Earlier work in 2005 revealed that GRETCHEN HAGEN 3 (GH3) proteins, known for their role in forming IAA-amides with amino acids (IAA-AAs), also exhibit in vitro sensitivity to PAA. To investigate the spectrum activity of GH3 enzymes to form PAA amino acid conjugates, recombinant AtGH3.6 and AtGH3.17 enzymes were tested with PAA using a bacterial assay. Nonetheless, AtGH3.6 predominantly conjugated PAA with Asp and AtGH3.17 with Glu. To understand the basis for amino acid specificity in GH3s, we solved the crystal structure of AtGH3.6 in the presence of AMP only or AMP together with aspartate, up to 1.74 Å resolution.

Superposition of both structures did not reveal rearrangement in the presence of amino acid (aspartate) ligand in the active site. Binding affinities for AtGH3.6 were analysed by MST. Affinities for IAA and PAA were similar and at around 60 µM concentration. The superposition of AtGH3.6 with AtGH3.5 shows the conservation of the amino acid binding site and, thus, similar specificity. Our attempts to obtain structures with bound products IAA-Asp or PAA-Asp were unsuccessful due to solubility issues of these ligands and a loss of crystal diffraction upon co-crystallization with AtGH3.6.

>[2x]MHHHHHHAMPEAPKIAALEVSDESLAEKNKNKLQFIEDVTTNADDVQRRVLEEILSRNADVEYLKRHGLEGRTDRETFKHIMPVVTYEDIQPEINRIANGDKSQVLCSNPISEFLTSSGTSGGERKLMPTIEEELDRRSLLYSLLMPVMDQFVPGLDKGKGMYFLFIKSESKTPGGLPARPVLTSYYKSSHFKNRPYDPYTNYTSPNQTILCSDSYQSMYSQMLCGLCQHKEVLRVGAVFASGFIRAIKFLEKHWPELARDIRTGTLSSEITDSSVREAVGEILKPDPKLADFVESECRKTSWQGIITRLWPNTKYVDVIVTGTMSQYIPTLDYYSNGLPLVCTMYASSECYFGVNLRPLCKPSEVSYTLIPNMAYFEFLPVHRNSGVTSSISLPKALTEKEQQELVDLVDVKLGQEYELVVTTYAGLYRYRVGDVLSVAGFKNNAPQFSFICRKNVVLSIDSDKTDEVELQNAVKNAVTHLVPFDASLSEYTSYADTSSIPGHYVLFWELCLNGNTPIPPSVFEDCCLTIEESLNSVYRQGRVSDKSIGPLEIKMVESGTFDKLMDYAISLGASINQYKTPRCVKFAPIIELLNSRVVDSYFSPKCPKWSPGHKQWGSN lipopolysaccharide fragment | C95 H182 N2 O25 P2 | 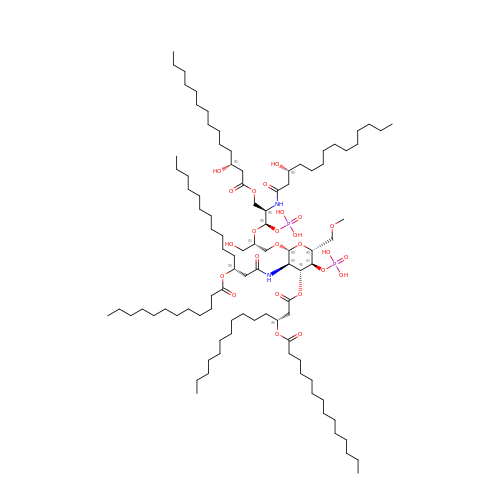WFPYFXOOZWPZCO-PICFCIIGSA-N>[10x]ESRTKPFTVPILTVEEMTNSRFPIPLEKLFTGPSSAFVVQPQNGRCTTDGALLGTTQLSPVDICTFRGDVTHIAGTQNYTMNLASQNWNNYDPTEEIPAPLGTPDFVGKIQGVL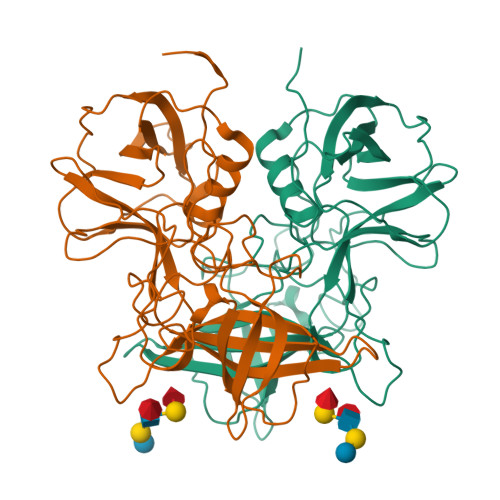TQTTRRDGSTRGHKATVSTGSVHFTPKLGSVQFSTDTSNDFETGQNTRFTPVGVVQDGSTTHQNEPQQWVLPDYSGRDSHNVHLAPAVAPTFPGEQLLFFRSTMPGCSGYPNMNLDCLLPQEWVQHFYQESAPAQSDVALLRFVNPDTGRVLFECKLHKSGYVTVAHTGQHDLVIPPNGYFRFDSWVNQFYTLAPMG> GSGPIQLWQFLLELLT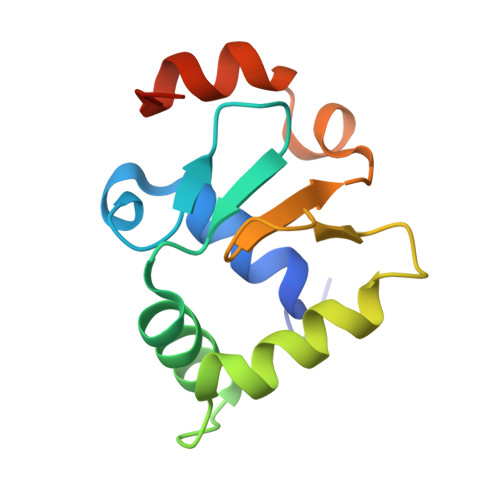DKSCQSFISWTGDGWEFKLSDPDEVARRWGKRKNKPKMNYEKLSRGLRYYYDKNIIHKTAGKRYVYRFVCDLQSLLGYTPEELHAMLDVKPDADE>[2x]SNARTTTYDVFLSFRGEDTRYNFTDHLYSALGRRGIRTFRDDRLRRGEAIAPELLKAIEESRSSVIVFSENYAHSRWCLDELVKIMECQKDLGHAVFPIFYHVDPSHVRKQEGSFGEAFAGYEENWKDKIPRWRTALTEAANLSGWHLLDDRYESNQIKEITNSIFRQLKCKRLDVG

M. rotundifolia is a wild North American grape species closely related to the cultivated grapevine species Vitis vinifera, and RPV1 confers resistance to the oomycete Plasmopara viticola, the casual agent of downy mildew in cultivated grapevines. The RPV1 gene from M. rotundifolia encodes a TIR-NB-LRR protein that confers resistance to the oomycte pathogen P. viticola. The multi-domain architecture of plant NLRs generally involves a C-terminal leucine-rich repeat (LRR) domain, a central nucleotide-binding (NB) domain and either a coiled-coil (CC) domain or Toll-interleukin receptor (TIR) domain at the N-terminus. Toll-interleukin receptor domains are protein scaffolds that regulate pathogen defense-related pathways in plants and animals through TIR:TIR domain interactions.

Here we report the crystal structure of the TIR domain of RPV1 (residues 20–193; RPV1TIR20-193) at 2.3 Å resolution. Within the asymmetric unit, we observe a dimer that resembles the heterodimer of the TIR domains from Arabidopsis RRS1 and RPS4. This interaction involves the αA and αE helices and the loop regions that precede both helices; we consequently define this protein-protein interface as the AE interface. Analysis of the RPV1TIR structure using the program PISA identified that the AE interface was the largest crystal lattice contact, contributing a combined buried surface area of ∼1340 Å2 (∼670 Å2 from each molecule). Within the AE interface, 17 surface-exposed amino-acids from each RPV1TIR20-193 monomer are buried within the dimer and contribute to the interaction. At the core of the interface, His42 forms an important stacking interaction between the two monomers and hydrogen bonds with Glu170 from the opposing monomer. Hydrogen bonding between Asp41 and Ser171 is also prominent and these equivalent residues were also important in the RPS4TIR:RRS1TIR interaction. Mutations of residues His42 and Asp41 to alanine within the core of the AE interface, were found to abolish and markedly reduce, RPV1TIR1-193-YFP mediated cell death in tobacco. In the case of RPV1TIR20-193, biophysical characterisation suggests that self-association, is absent or very weak in solution. An interesting feature of the cell death induced by RPV1 is that the region that encompasses the TIR domain structure is, itself, sufficient to induce cell death.> DDFRVGERVWVNGNKPGFIQFLGETQFAPGQWAGIVLDEPIGKNDGSVAGVRYFQCEPLKGIFTRPSKLTR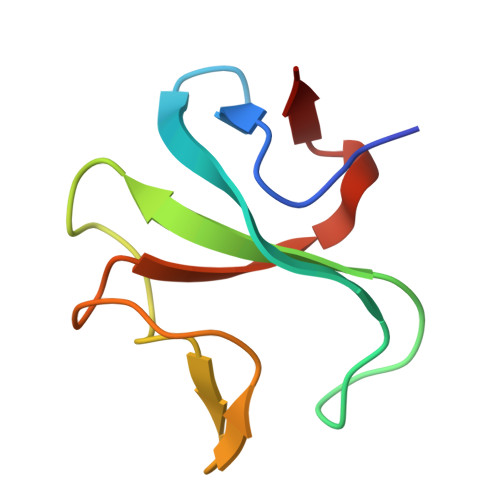K> MQLNATFYSGTCPNASAIVRSTIQQALQSDTRIGASLIRLHFHDCFVNGCDASILLDDTGSIQSEKNAGPNVNSARGFNVVDNIKTALENACPGVVSCSDVLALASEASVSLAGGPSWTVLLGRRDSLTANLAGANSSIPSPIESLSNITFKFSAVGLNTNDLVALSGAHTFGRARCGVFNNRLFNFSGTGNPDPTLNSTLL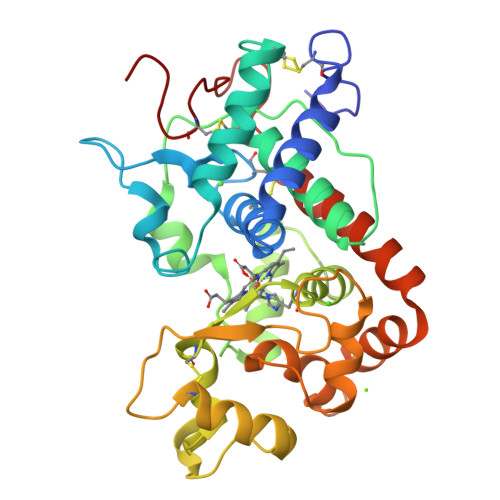STLQQLCPQNGSASTITNLDLSTPDAFDNNYFANLQSNDGLLQSDQELFSTTGSSTIAIVTSFASNQTLFFQAFAQSMINMGNISPLTGSNGEIRLDCKKVNGS5-(4-METHYL-BENZOYLAMINO)-BIPHENYL-3,4'-DICARBOXYLIC 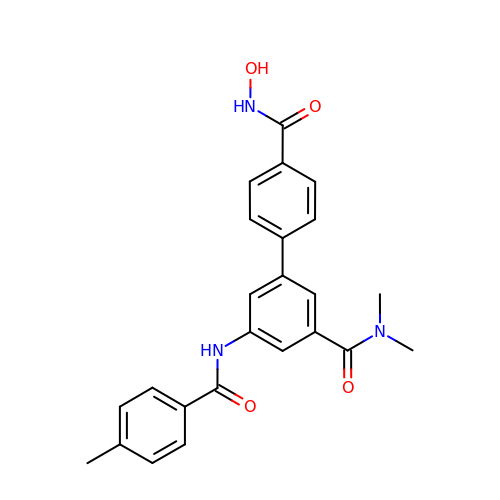ACID 3-DIMETHYLAMIDE-4'-HYDROXYAMIDE | C24 H23 N3 O4 | DOPFUKKMSDUVTQ-UHFFFAOYSA-N>[2x]RPEKPVYLSVKADNSMFIG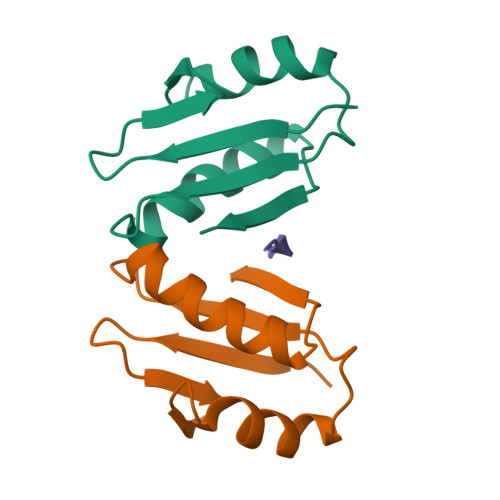NDPVTDETMITALNALTEGKKDTTIFFRADKTVDYETLMKVMDTLHQAGYLKIGLVGEETAKAK;> QPISVTMVT>MRSYDMNVETAAELSAVNDILASIGEPPVSTLEGDANADAANARRILNKINRQIQSRGWTFNIEEGITLLPDVYSNLIVYSDDYLSLMSTSGQSIYVNRGGYVYDRTSQSDRFDSGITVNIIRLRDYDEMPECFRYWIVTKASRQFNNRFFGAPEVEGVLQEEEDEARRLCMEYEMDYGGYNMLDGDAFTSGLLTR[2x];>[3x]MANVIKTVLTYQLDGSNRDFNIPFEYLARKFVVVTLIGVDRKVLTINTDYRFATRTTISLTKAWGPADGYTTIELRRVTSTTDRLVDFTDGSILRAYDLNVAQIQTMHVAEEARDLTTDTIGVNNDGHLDARGRRIVNLANAVDDRDAVPFGQLKTMNQNSWQAR;> MALISQSIKNLKGGISQQPDILRYPDQGSRQVNGWSSETEGLQKRPPLVFLNTLGDNGALGQAPYIHLINRDEHEQYYAVFTGSGIRVFDLSGNEKQVRYPNGSNYIKTANPRNDLRMVTVADYTFIVNRNVVAQKNTKSVNLPNYNPNQDGLINVRGGQYGRELIVHINGKDVAKYKIPDGSQPEHVNNTDAQWLAEELAKQMRTNLSDWTVNVGQGFIHVTAPSGQQIDSFTTKDGYADQLINPVTHYAQSFSKLPPNAPNGYMVKIVGDASKSADQYYVRYDAERKVWTETLGWNTEDQVLWETMPHALVRAADGNFDFKWLEWSPKSWGDVDTNPWPSFVGSSINDVFFFRNRLGFLSGENIILSRTAKYFNFYPASIANLSDDDPIDVAVSTNRIAILKYAVPFSEELLIWSDEAQFVLTASGTLTSKSVELNLTTQFDVQDRARPFGIGRNVYFASPRSSFTSIHRYYAVQDVSSVKNAEDITSHVPNYIPNGVFSICGSGTENFCSVLSHGDPSKIFMYKFLYLNEELRQQSWSHWDFGENVQVLACQSISSDMYVILRNEFNTFLARISFTKNAIDLQGEPYRAFMDMKIRYTIPSGTYNDDTFTTSIHIPTIYGANFGRGKITVLEPDGKITVFEQPTAGWNSDPWLRLSGNLEGRMVYIGFNINFVYEFSKFLIKQTADDGSTSTEDIGRLQLRRAWVNYENSGTFDIYVENQSSNWKYTMAGARLGSNTLRAGRLNLGTGQYRFPVVGNAKFNTVYILSDETTPLNIIGCGWEGNYLRRSSGI;> GQNAQAKMIAAQTAAGRRQAMEIMRQTNIQNADLSLQARSKLEEASAELTSQNMQKVQAIGSIRAAIGESMLEGSSMDRIKRVTEGQFIREANMVTENYRRDYQAIFAQQLGGTQSAASQIDEIYKS;>[2x]MAEKRTGLAEDGAKSVYERLKNDRAPYETRAQNCAQYTIPSLFPKDSDNASTDYQTPWQAVGARGLNNLASKLMLALFPMQTWMRLTISEYEAKQLLSDPDGLAKVDEGLSMVERIIMNYIESNSYRVTLFEALKQLVVAGNVLLYLPEPEGSNYNPMKLYRLSSYVVQRDAFGNVLQMVTRDQIAFGALPEDIRKAVEGQGGEKKADETIDVYTHIYLDEDSGEYLRYEEVEGMEVQGSDGTYPKEACPYIPIRMVRLDGESYGRSYIEEYLGDLRSLENLQEAIVKMSMISSKVIGLVNPAGITQPRRLTKAQTGDFVTGRPEDISFLQLEKQADFTVAKAVSDAIEARLSFAFMLNSAVQRTGERVTAEEIRYVASELEDTLGGVYSILSQELQLPLVRVLLKQLQATQQIPELPKEAVEPTISTGLEAIGRGQDLDKLERCVTAWAALAPMRDDPDINLAMIKLRIANAIGIDTSGILLTEEQKQQKMAQQS;> MSKIESALQAAQPGLSRLRGGAGGMGYRAATTQAEQP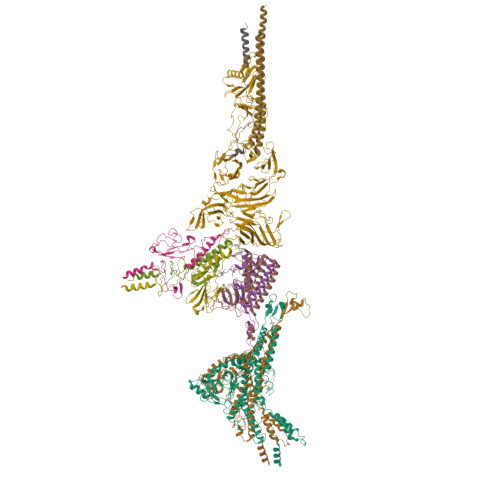RSSLLDTIGRFAKAGADM>GAMENQAPVANFELKTDGLSVSAFNYSHDEDGELVSYAWDFGNGQMSSEMAPSWSYTRAGQYTVSLTVTDDKGATNTTTRTTQVEV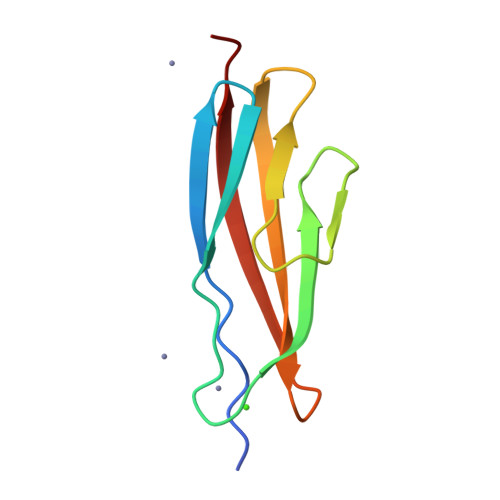P[2x]>SNAMKFLELNKKRHATKHFTDKLVDPKDVRTAIEIATLAPSAHNSQPWK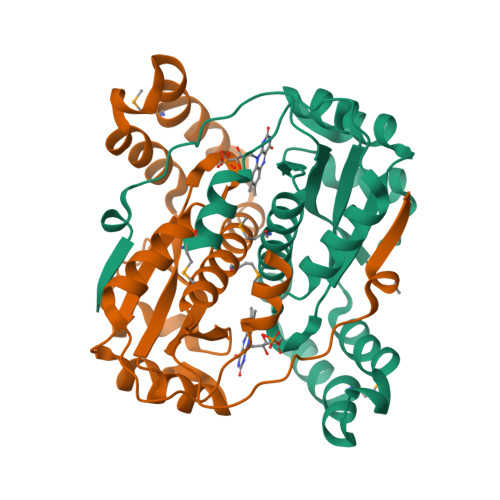FVVVREKNAELAKLAYGSNFEQVSSAPVTIALFTDTDLAKRARKIARVGGANNFSEEQLQYFMKNLPAEFARYSEQQVSDYLALNAGLVAMNLVLALTDQGIGSNIILGFDKSKVNEVLEIEDRFRPELLITVGYTDEKLEPSYRLPVDEIIEKR[4x]> SNAMSYPGKDKNIPGRIIEALEDLPLSYLVPKDGLAALVN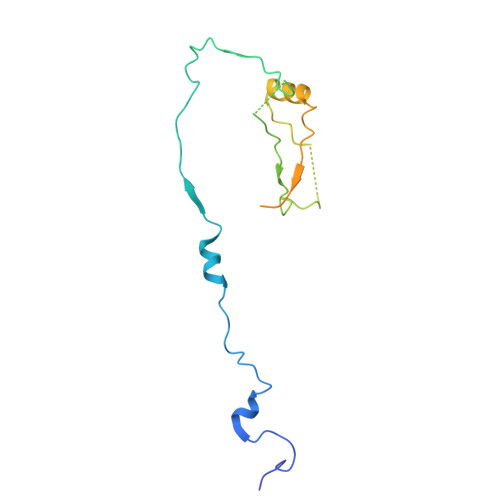APMRVSLPFDKTIFTSADDGRDVNINVLGTANSTTSSIKNEAEKERLVFKRPSNFTSSANSVDYVPTNFLEGLSPLAQSVLSTHKGLNDSINIEKKSEIVSRPEAKHKLESVTSNAGNLSFNDNSSNKKTKTSTGVTMTQANLA> MRSCRRSVAQHPCAIQVDIVAMAAFISSFAGAQLAHARPSKQTALRAALTLPGTAETNLAVPSNAVRKVQPYPIAKPPSYSSVDSLRPARVSRMDADWATIYEQVRRQVMGNAYVMEGEAPDIDVAFSQLKGGNLTVREFVRAVGKSASYRTRFMEAKSSYNFVLLNFKHFLGRAPTQEEVSTHIQILATSGLEAEIDSYIDSDEYKALFGDHVVPYVVYRGTYLSSERFNRMVKANPGGATSDKAKSNLNMIATVAADLPTDAIDVMRGLPSPITSETLAFGTAYYWAKVEKEASEGRSASPIGEKIGKFDHAPISTYTSLCSYDKVNKAPQISVTNVGSDEHSYVSVTSKYIAPDMAAAAQMLADCQKYKAGGNAPTGKWMKYYPGTTVNMAPYIS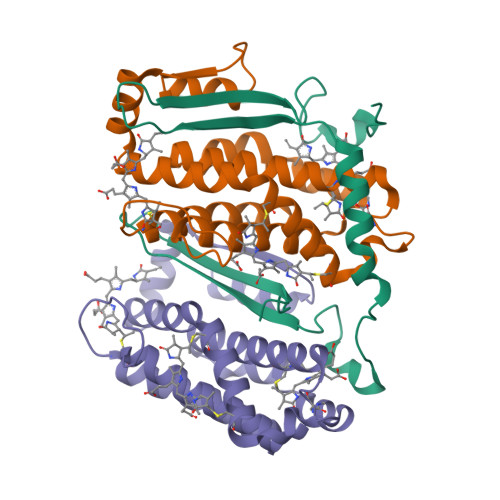LNDTGSDSSRTVSVTLDKVKISPNKIGK;>[2x]MLDAFSRVVVNSDAKAAYVGGSDLQALKSFIADGNKRLDAVNSIVSNASCMVSDAVSGMICENPGLISPGGNCYTNRRMAACLRDGEIILRYVSYALLAGDASVLEDRCLNGLKETYIALGVPTNSSIRAVSIMKAQAVAFITNTATERKMSFAAGDCTSLASEVASYFDRVGAAIS> GPTASGMDAELQGLLQATMARAKEVKDAEVFKLLKLMSWTRKNDLTDHMYEWSKEDPDAIKFGRLVSTPPKHQEKPKGPDQHTAQEAKATRISLDAVKAGADFASPEWIAENNYRGPSPGQFKYYMITGRVPNPGEEYEDYVRKPITRPTDMDKIRRLANSVYGLPHQEPAPDDFYQAVVEVFAENGGR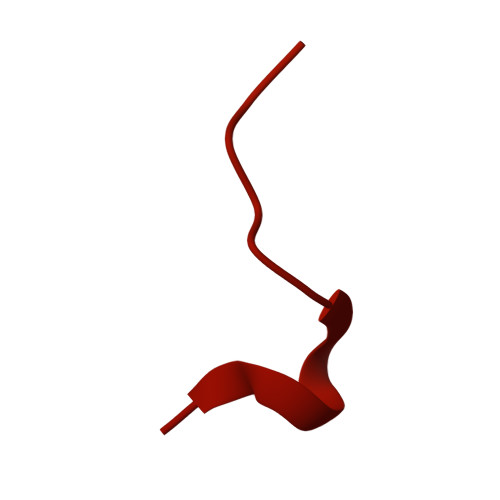GPDQDQMQDLRDLARQMKRRPRPAETRRQTKTPPRAATSSGSRFTPSGDDGEV>MSSKANHAKTVICGIINVTPDSFSDGGQFFALEQALQQARKLIAEGASMLDIGGESTRPGSSYVEIEEEIQRVVPVIKAIRKESDVLISIDTWKSQVAEAALAAGADLVNDITGLMGDEKMPHVVAEARAQVVIMFNPVMARPQHPSSLIFPHFGFGQAFTEEELADFETLPIEELMEAFFERALARAAEAGIAPENILLDPGIGFGLTKKENLLLLRDLDKLHQKGYPIFLGVSRKRFVINILEENGFEVNPETELGFRNRDTASAHVTSIAARQGVEVVRVHDVASHRMAVEIASAIRLADEAENLDLKQ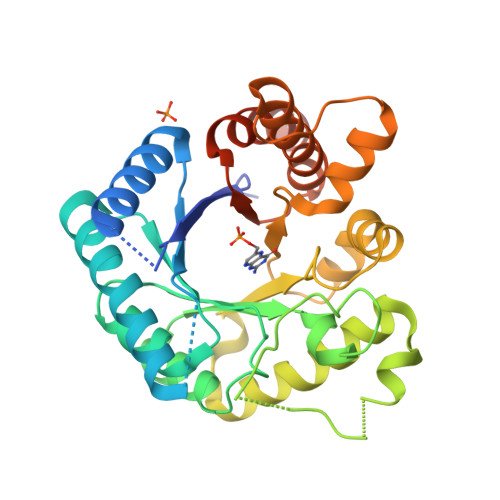YK[2x]> MKKLTGLIAAPHTPFDSSSNVNFEEIDKIAKHLINDGVKGIYVCGTTGEGIHCSVEERKAIAERWVSACNHKLDIIVHTGALSIVDTLELTRHADTLDILATSAIGPCFFKPGSVSDLVEYCATIAAAAPSKGFYYYHSGMSGVNLNMEEFLIQADKRIPNLSGLKFNSGDLYEYQRCLRACDGKFDVPFGVDEFLPGALAVGAKSAVGSTYNYAAP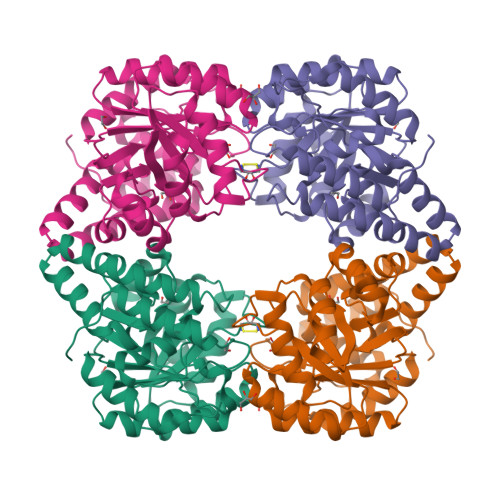HFNSIIEAFNKGDHDAVFNKMTNVIELIRVLVEFGGVAAGKIAMELHDINAGDPRLPLMPLSAEQKLTVVEKMRAANFLKHHH>MALSKVKLNDTLNKDQLLSSSKYTIQRSTGD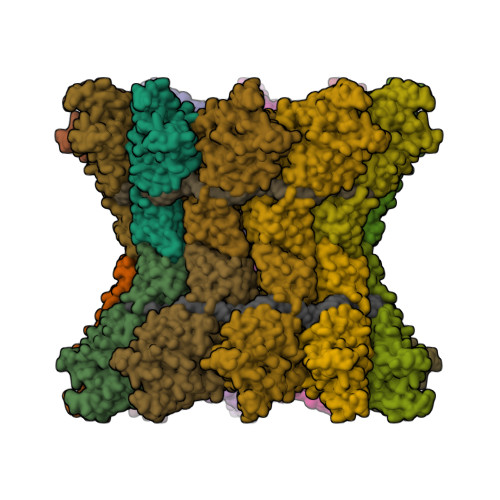SIDTPNYDVQKHINKLCGMLLITEDANHKFTGLIGMLYAMSRLGREDTIKILRDAGYHVKANGVDVTTHRQDINGKEMKFEVLTLASLTTEIQINIEIESRKSYKKMLKEMGEVAPEYRHDSPDCGMIILCIAALVITKLAAGDRSGLTAVIRRANNVLKNEMKRYKGLLPKDIANSFYEVFEKHPHFIDVFVHFGIAQSSTRGGSRVEGIFAGLFMNAYGAGQVMLRWGVLAKSVKNIMLGHASVQAEMEQVVEVYEYAQKLGGEAGFYHILNNPKASLLSLTQFPHFSSVVLGNAAGLGIMGEYRGTPRNQDLYDAAKAYAEQLKENGVINYSVLDL[20x]N-[5-(3,6-dihydro-2H-pyran-4-yl)-2-methoxy-pyridin-3-yl]benzenesulfonamide | C17 H18 N2 O4 S | 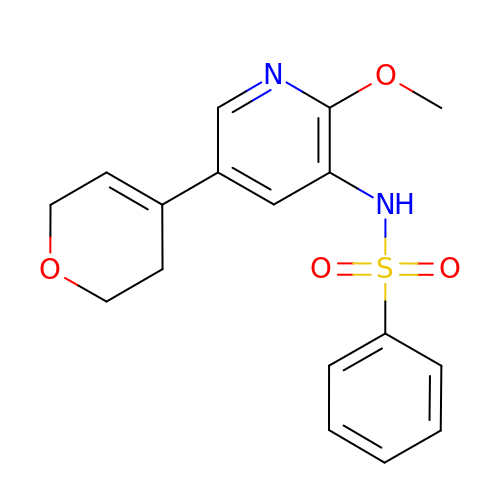OZEVUWLUKNYTLV-UHFFFAOYSA-N> ADYIEMKVPAQPEYVGIIRLTLSGVASRMGYTYDEIEDLKIAVSEACTNAVQHAYKEDKNGEVSIRFGVFEDRLEVIVADEGDSFDFDQKQQDLGP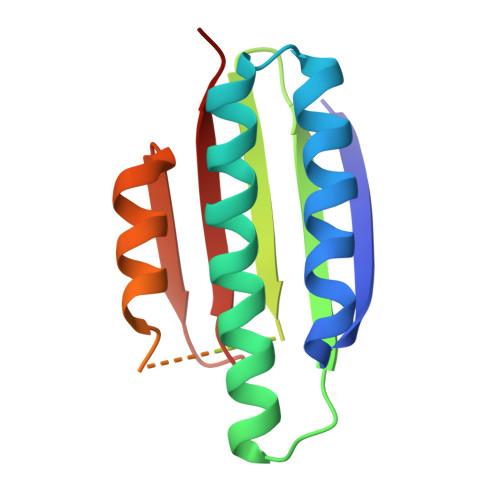YTPSHTVDQLSEGGLGLYLMETLMDEVRVQNHSGVTVAMTKYLNG> IVGGYTCGANTVPYQVSLNSGYHFCGGSLINSQWVVSAAHCYKSGIQVRLGCDNINVVEGNCQFISASKSIVHPSYNSNTLNNDIMLIKLKSAASLNSRVASISLPTSCASAGTQCLISGWGNTKSSGTSYPDVLKCLKAPILSDSSCKSAYPGQI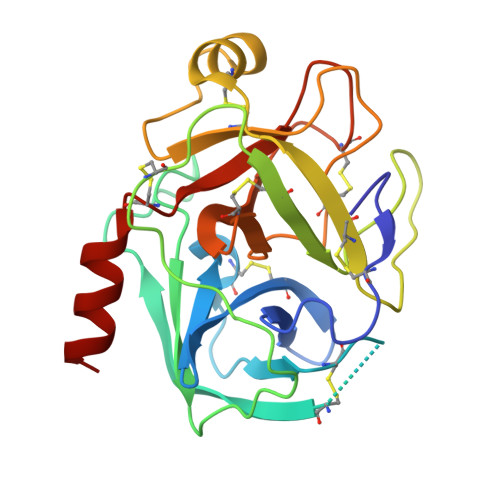TSNMFCAGYLEGGKDSCQGDAGGPVVCSGKLQGIVSWGSGCAQKNKPGVYTKVCNYVSWIKQTIASN>[4x]MADRTGIVAGALLPGMPHLLAEHPAPSWSALAGAARDVGARLRRLEPDVVLLLSTQWFTVLGHQFQCDPNPRGEHVDENWYAYDYGLLDYDLRFDVDFTERWADRVQAGGMQARRTRYDGFPIDTGTIVTSALLDPDRRLRWAQVSCNLYADADTLADVGRAGAAAARDAGLRAAVVVVTGMSSGLIQQWIEPGQDRIGEPGHDQWNTRVLDLLTAGKVDEVLAVREDFARQAQADSQFRALAFAAGAEATTGPAHLHAYGPIWGTGAAVLSWNLPDHP;>[4x]MSRVFRVPLAPTRGGATTAPRTPAPAPAPTRPGIVAGCLSPHPPHLIYGENPPQNEPRSTGGWETLRWAYERLRARIRDVHKPD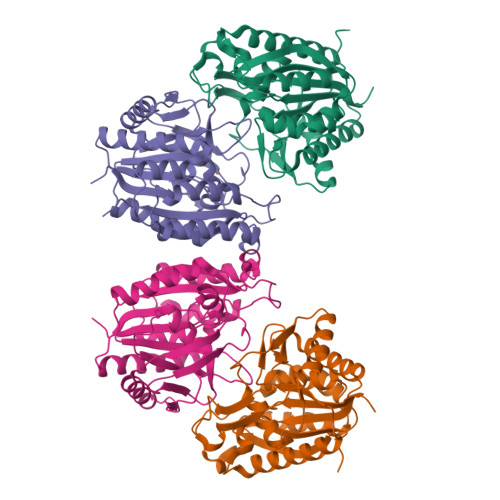VLIVHAPHWITMVGHHVNCVPNPRGLSVEPIFPHLFRYRYDFRTDVELGEAIAEEASGLGLVTRTLRDPRVRVDYATIGALHLANPAWDIPVVSLSANNNPYFYSDASLTEMEVLGEATRLAVEATGRRAVLLASNSLSHLHWHEEPELPEDMEREHPYNNHQYRWDMKLLEAIRRGPTAPLRDLIPEHIEATASETKAGSLTWMLAAMGWPKVAGDVLGYGTIIGTGNAIVEWLPEGSHHGGSGGSHHHHHH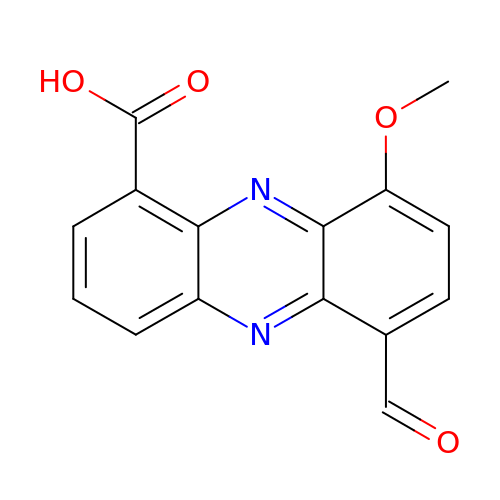6-formyl-9-methoxyphenazine-1-carboxylic acid | C15 H10 N2 O4 | NJJLLHHIAVHAEL-UHFFFAOYSA-N> GPHMLEREKIYQWINELSSPETRENALLELSKKRESVPDLAPMLWHS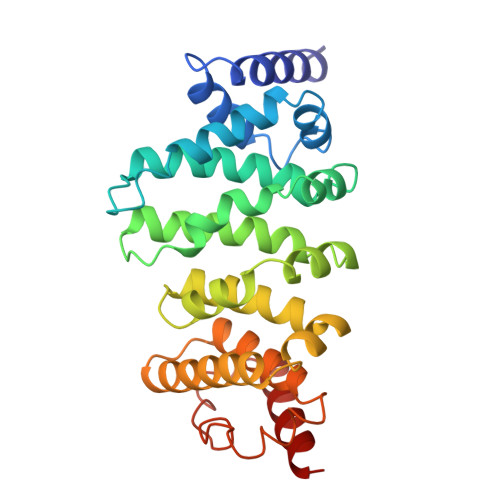FGTIAALLQEIVNIYPSINPPTLTAHQSNRVCNALALLQCVASHPETRSAFLAAHIPLFLYPFLHTVSKTRPFEYLRLTSLGVIGALVKTDEQEVINFLLTTEIIPLCLRIMESGSELSKTVATFILQKILLDDTGLAYICQTYERFSHVAMILGKMVLQLSKEPSARLLKHVVRCYLRLSDNPRAREALRQCLPDQLKDTTFAQVLKDDTTTKRWLAQLVKNLQE> SNALEDAQESKALVNMPGPSSESLGKDDKPISLQNWKRGLDILSPMERFHLKYLYVTDLAEQNWCELQTAYGKELPGFLAPEKAAVLDTGASIHLARELELHDLVTVPVTTKEDAWAIKFLNILLLIPTLQSEGHIREFPVFGEVEGVLLVGVIDELHYTAKGELELAELKTRRRPMLPLEAQKKKDCFQVSLYKYIFDAMVQGKVTPASLIHHTKLCLEKPLGPSVLRHAQQGGFSVKSLGDLMELVFLSLTLSDLPVIDILKIEYIHQETATVLGTEIVAF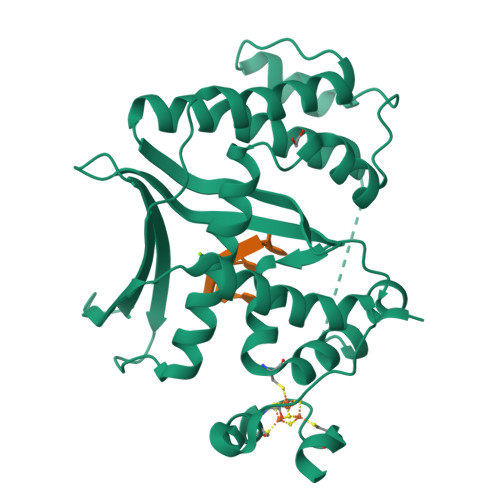KEKEVRAKVQHYMAYWMGHREPQGVDVEEAWKCRTCTYADICEWRKGSGVLSSTLAPQVKKAK> MDAATTRVGLTDLTFRLLRESFADAVSWVAKNLPARPAVPVLSGVLLTGSDNGLTISGFDYEVSAEAQVGAEIVSPGSVLVSGRLLSDITRALPNKPVDVHVEGNRVALTCGNARFSLPTMPVEDYPTLPTLPEETGLLPAELFAEAISQVAIAAGRDDTLPMLTGIRVEILGETVVLAATDRFRLAVRELKWSASSPDIEAAVL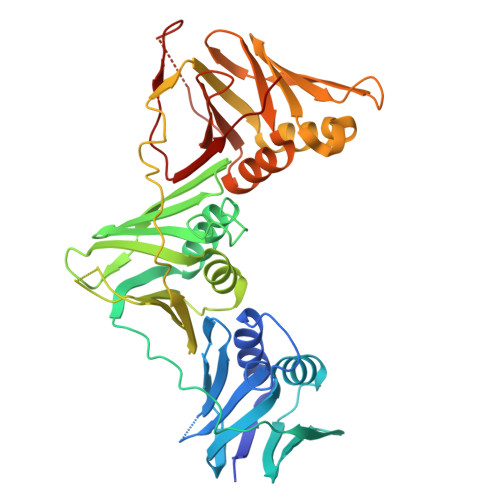VPAKTLAEAAKAGIGGSDVRLSLGTGPGVGKDGLLGISGNGKRSTTRLLDAEFPKFRQLLPTEHTAVATMDVAELIEAIKLVALVADRGAQVRMEFADGSVRLSAGADDVGRAEEDLVVDYAGEPLTIAFNPTYLTDGLSSLRSERVSFGFTTAGKPALLRPVSGDDRPVAGLNGNGPFPAVSTDYVYLLMPVRLPG>MIVLFVDFDYFYAQVEEVLNPSLKGKPVVVCVFSGRFEDSGAVATANYEARKFGVKAGIPIVEAKKILPNAVYLPMRKEVYQQVSSRIMNLLREYSEKIEIASIDEAYLDISDKVRDYREAYNLGLEIKNKILEKEKITVTVGISKNKVFAKIAADMAKPNGIKVIDDEEVKRLIRELDIADVPGIGNITAEKLKKLGINKLVDTLSIEFDKLKGMIGEAKAKYLISLARDEYNEPIRTRVRKSIGRIVTMKRNSRNLEEIKPYL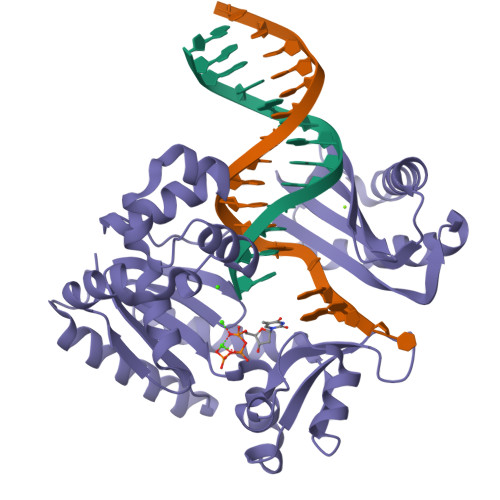FRAIEESYYKLDKRIPKAIHVVAVTEDLDIVSRGRTFPHGISKETAYSESVKLLQKILEEDERKIRRIGVRFSKFIEAIGLDKFFDT[2x]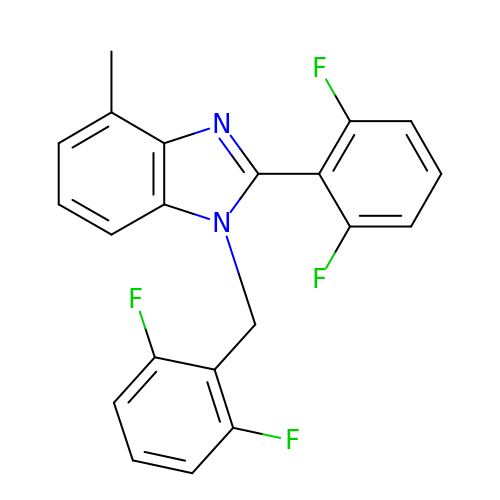1-(2,6-DIFLUOROBENZYL)-2-(2,6-DIFLUOROPHENYL)-4-METHYL-1H-BENZIMIDAZOLE | C21 H14 F4 N2 | JIYRSPUMGRIYBL-UHFFFAOYSA-N> MALVYDAEFVGSEREFEEERETFLKGVKAYDGVLATRYLMERSSSAKNDEELLELHQNFILLTGSYACSIDPTEDRYQNVIVRGVNFDERVQRLSTGGSPARYAIVYRRGWRAIAKALDIDEEDVPAIEVRAVKRNPLQPALYRILVRYGRVDLMPVTVDEVPPEMAGEFERLIERYDVPIDEKEERILEILRENPWTPHDEIARRLGLSVSEVEGEKDPESSGIYSLWSRVVVNIEYDERTAKRHVKRRDRLLEELYEHLEELSERYLRHPLTRRWIVEHKRDIMRRYLEQRIVECALKLQDRYGIREDVALCLARAFDGSISMIATTPYRTLKDVCPDLTLEEAKSVNRTLATLIDEHGLSPDAADELIEHFESIAGILATDLEEIERMYEEGRLSEEAYRAAVEIQLAELTKKEGVGRKTAERLLRAFGNPERVKQLAREFEIEKLASVEGVGERVLRSLVPGYASLISIRGIDRERAERLLKKYGGYSKVREAGVEELREDGLTDAQIRELKGLKTLESIVGDLEKADELKRKYGSASAVRRLPVEELRELGFSDDEIAEIKGIPKKLREAFDLETAAELYER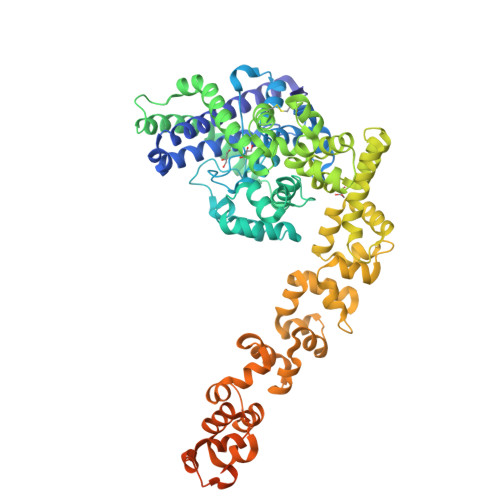YGSLKEIGRRLSYDDLLELGATPKAAAEIKGPEFKFLLNIEGVGPKLAERILEAVDYDLERLASLNPEELAEKVEGLGEELAERVVYAARERVESRRK> GPGSMKQYVARLEKDFSLIEHGFKEEEQRALTDYKSNDGEYIKKLAFLAYQSDVYQVRMYAVFLFGYLSKDKE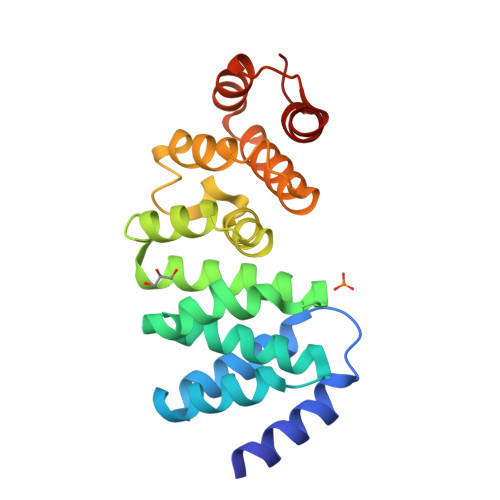ILIFMRDEVSKDNNWRVQEVLAKAFDEFCKKIGYKKALPIIDEWLKSSNLHTRRAATEGLRIWTNRPYFKENPNEAIRRIADLKEDVSEYVRKSVGNALRDISKKFPDLVKIELKNWKLESKEINQVYKLASKFIDA> MAHHHHHHSNSDAAHAFWSTQPVPQTEDETEKIVFAGPMDEPKTVADIPEEPYPIASTFEWWTPNMEAADDIHAIYELLRDNYVEDDDSMFRFNYSEEFLQWALCPPNYIPDWHVAVRRKADKKLLAFIAGVPVTLRMGTPKYMKVKAQEKGEGEEAAKYDEPRHICEINFLCVHKQLREKRLAPILIKEA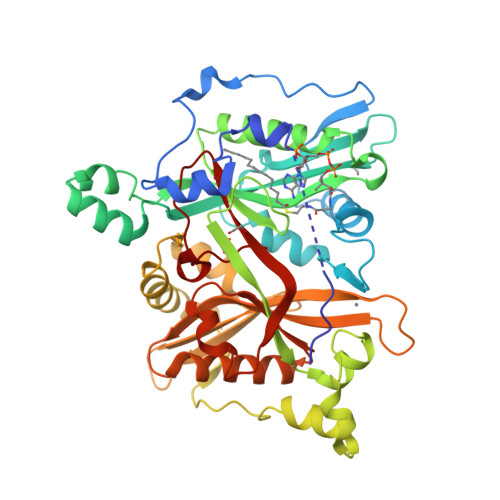TRRVNRTNVWQAVYTAGVLLPTPYASGQYFHRSLNPEKLVEIRFSGIPAQYQKFQNPMAMLKRNYQLPSAPKNSGLREMKPSDVPQVRRILMNYLDSFDVGPVFSDAEISHYLLPRDGVVFTYVVENVKKVTDFFSFYRIPSTVIGNSNYNLLNAAYVHYYAATSIPLHQLILDLLIVAHSRGFDVCNMVEILDNRSFVEQLKFGPGDGHLRYYFYNWAYPKIKPSQVALVML> MKLPLLLALLFGAVSALHLRSETSTFETPLGAKTLPEDEETPEQEMEETPCRELEEEEEWGSGSEDASKKDGAVESISVPDMVDKNLTCPEEEDTVKVVGIPGCQTCRYLLVRSLQTFSQAWFTCRRCYRGNLVSIHNFNINYRIQCSVSALNQGQVWIGGRITGSGRCRRFQWVDGSRWNFAYWAAHQPWSRGGHCVALCTRGGHWRRAHCLRRLPFICSY;>[2x]REARGATEEPSPPSRALYFSGRGEQLRLRADLELPRDAFTLQVWLRAEGGQRSPAVITGLYDKCSYISRDRGWVVGIHTISDQDNKDPRYFFSLKTDRARQVTTINAHRSYLPGQWVYLAATYDGQFMKLYVNGAQVATSGEQVGGIFSPLTQKCKVLMLGGSALNHNYRGYIEHFSLWKVARTQREILSDMETHGAHTALPQLLLQENWDNVKHAWSPMKDGSSPKVEFSNAHGFLLDTSLEPPLCGQTLCDNTEVIASYNQLSSFRQPKVVRYRVVNLYEDDHKNPTVTREQVDFQHHQLAEAFKQYNISWELDVLEVSNSSLRRRLILANCDISKIGDENCDPECNHTLTGHDGGDCRHLRHPAFVKKQHNGVCDMDCNYERFNFDGGECCDPEITNVTQTCFDPDSPHRAYLDVNELKNILKLDGSTHLNIFFAKSSEEELAGVATWPWDKEALMHLGGIVLNPSFYGMPGHTHTMIHEIGHSLGLYHVFRGISEIQSCSDPCMETEPSFETGDLCNDTNPAPKHKSCGDPGPGNDTCGFHSFFNTPYNNFMSYADDDCTDSFTPNQVARMHCYLDLVYQGWQPSRKPAPVALAPQVLGHTTDSVTLEWFPPIDGHFFERELGSACHLCLEGRILVQYASNASSPMPCSPSGHWSPREAEGHPDVEQPCKSSVRTWSPNSAVNPHTVPPACPEPQGCYLELEFLYPLVPESLTIWVTFVSTDWDSSGAVNDIKLLAVSGKNISLGPQNVFCDVPLTIRLWDVGEEVYGIQIYTLDEHLEIDAAMLTSTADTPLCLQCKPLKYKVVRDPPLQMDVASILHLNRKFVDMDLNLGSVYQYWVITISGTEESEPSPAVTYIHGSGYCGDGIIQKDQGEQCDDMNKINGDGCSLFCRQEVSFNCIDEPSRCYFHDGDGVCEEFEQKTSIKDCGVYTPQGFLDQWASNASVSHQDQQCPGWVIIGQPAASQVCRTKVIDLSEGISQHAWYPCTISYPYSQLAQTTFWLRAYFSQPMVAAAVIVHLVTDGTYYGDQKQETISVQLLDTKDQSHDLGLHVLSCRNNPLIIPVVHDLSQPFYHSQAVRVSFSSPLVAISGVALRSFDNFDPVTLSSCQRGETYSPAEQSCVHFACEKTDCPELAVENASLNCSSSDRYHGAQCTVSCRTGYVLQIRRDDELIKSQTGPSVTVTCTEGKWNKQVACEPVDCSIPDHHQVYAASFSCPEGTTFGSQCSFQCRHPAQLKGNNSLLTCMEDGLWSFPEALCELMCLAPPPVPNADLQTARCRENKHKVGSFCKYKCKPGYHVPGSSRKSKKRAFKTQCTQDGSWQEGACVPVTCDPPPPKFHGLYQCTNGFQFNSECRIKCEDSDASQGLGSNVIHCRKDGTWNGSFHVCQEMQGQCSVPNELNSNLKLQCPDGYAIGSECATSCLDHNSESIILPMNVTVRDIPHWLNPTRVERVVCTAGLKWYPHPALIHCVKGCEPFMGDNYCDAINNRAFCNYDGGDCCTSTVKTKKVTPFPMSCDLQGDCACRDPQAQEHSRKDLRGYSHG

Originally discovered in the circulation of pregnant women as a protein secreted by placental trophoblasts, the metalloprotease pregnancy-associated plasma protein A (PAPP-A) is also widely expressed by many other tissues. It cleaves insulin-like growth factor-binding proteins (IGFBPs) to increase the bioavailability of IGFs and plays essential roles in multiple growth-promoting processes. While the vast majority of the circulatory PAPP-A in pregnancy is proteolytically inactive due to covalent inhibition by proform of eosinophil major basic protein (proMBP), the activity of PAPP-A can also be covalently inhibited by another less characterized modulator, stanniocalcin-2 (STC2). Here we present two cryo-EM structures of endogenous purified PAPP-A in complex with either proMBP or STC2. Both modulators form 2:2 heterotetramer with PAPP-A and establish extensive interactions with multiple domains of PAPP-A that are distal to the catalytic cleft.

To assess the molecular mechanism(s) subserving PAPP-A activity and the modulation of proMBP, we purified endogenous PAPP-A·proMBP complex from pregnant human plasma and determined its cryo-EM structure. The cryo-EM analysis generated an initial dimeric 3D map at 3.64 Å resolution, and C2-symmetry expansion was subsequently applied to obtain a final 3.45-Å monomeric half map, which enabled de novo modeling of most of the PAPP-A residues. The density at the interface between proMBP and PAPP-A was sufficiently resolved to analyze the detailed interaction. Besides, plenty of glycosylation sites could be unambiguously assigned, and a few coordinated Ca2+ ions could be identified. The structure not only confirmed intramolecular disulfide bonds of PAPP-A reported in previous studies, but also identified several new disulfide pairs. In addition to the previously reported covalent linkage between PAPP-A-Cys652 and proMBP-Cys16932, we also found that several other residues of PAPP-A in this region, such as Asn683 and His689, contribute to the stabilization of this interface. In the PAPP-A·proMBP complex, the binding of proMBP induces a nearly 30° rotation of the βBD towards the PD, generating an interface between the βBD and the C-terminal subdomain of PD. The mature form of proMBP is known to bind heparin; and in the PAPP-A·proMBP complex, this binding site is partially blocked by the CTD interaction.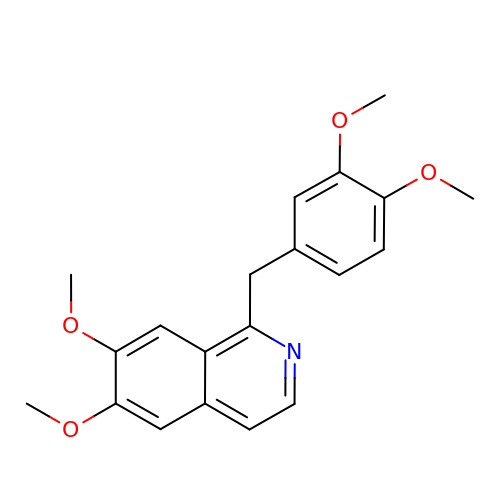1-(3,4-DIMETHOXYBENZYL)-6,7-DIMETHOXYISOQUINOLINE | C20 H21 N O4 | XQYZDYMELSJDRZ-UHFFFAOYSA-N>GPGSMNETLYGDGAIRRPSVYGSSIENTYAGVLSFMRRNYTRDLDGVDVVVSGVPLDLATTFRSGARLGPSAVRAASVQLAELNPYPWGFDPFDDLAVIDYGDCWFDAHHPLSIKPAIVEHARTILQSDARMLTLGGDHYITYPLLIAHAQKYGKPLSLIHFDAHCDTWADDAPDSLNHGTMFYKAVKDGLIDPKASVQVGIRTWNDDYLGINVLDAAWVHEHGARATLERIESIVGGRPAYLTFDIDCLDPAFAPGTGTPVAGGLSSAQALAIVRGLGGVNLIGADVVEV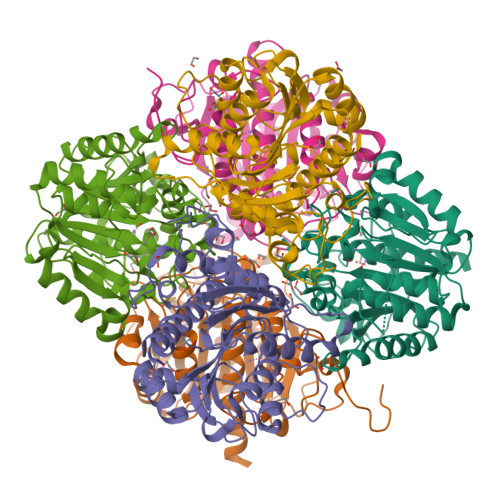APAYDQSEITAIAAAHVACDLLCLWRQRKAGAR[6x]The 2H phosphoesterase superfamily is an ancient group of proteins and protein domains characterized by a common fold and a few conserved active site residues. E. coli LigT is a 20-kDa protein that exhibits 2′,3′-cyclic nucleotide 3′-phosphodiesterase and 2′-5′-ligase/phosphodiesterase activities, but the biological function of the enzyme is unknown. The LigT structure presents a typical 2H phosphoesterase fold, in which the catalytic residues reside at the beginning of strands β2 and β6. As in other 2H family members, the active site has 2-fold symmetry; this symmetry also includes the 4 water molecules at the bottom of the active site, connecting the active-site β strands through water-mediated hydrogen bonds.

Another product analogue of the reaction catalysed by LigT, NADP+, was also trapped in the active site, being well defined in electron density. In the NADP+ complex, there are 4 monomers in the asymmetric unit, and the nicotinamide end of the ligand binds to each of them differently, having different conformations or being disordered—depending on crystal contacts. The adenosine 2′,5′-bisphosphate moiety in each monomer binds identically, however, and in a mode highly similar to that seen in 2′-AMP. The 5′-phosphate mimics the next phosphodiester in an RNA molecule, and it can be used to deduce further binding determinants for RNA substrates. This phosphate moiety is bound by Arg6 from the N-terminal strand β1 in the crystal structure, and it is likely that this residue plays a direct role in RNA substrate binding also. An additional NADP+ fragment is seen stacked on top of Trp82 in one monomer. In the NADP+ complex, we actually observe unidentified electron density of a stacking interaction, modeled as a fragment of NADP+, on top of Trp82, which could reflect low-affinity binding of some moiety in NADP+. The orientation of the reaction products 2′-AMP and NADP+ in the active site indicates the direction, into which an RNA molecule would continue, considering the last residue sits in the active site.

>[4x]GMSEPQRLFFAIDLPAEIREQIIHWRAKHFPPEAGRPVAADNLHLTLAFLGEVSAEKEKALSLLAGRIRQPGFTLTLDDAGQWLRSRVVWLGMRQPPRGLIQLANMLRSQAARSGCFQSNRPFHPHITLLRDASEAVTIPPPGFNWSYAVTEFTLYASSFARGRTRYTPLKRWALTQ>[4x]MRNKIFISHATPDDNDFTRWLALKLIGLGYEVWCDILFLDKGVDFWSNIEKVIREDTCKFLLVSSSYSNQREGVLKELAVAAKVKKQLKDDKFIIPLAIDEQLSYDDINIDIVRLNAIDFKMSWARGLKDILEAFEKQKVPKEVADASKSNLLYQQIFLHDKSVIEKEEIYDSNWLSILSFPEELRFHEYNWMLPKRFDVRELTFPAVRYKNYLCTFAWAYDFTYHLPKTETYHKSKTIRIPTEEILSGSYDSNFIRNAECKRLIVQLLNKAFELRMKDKEVQEYEMSNKTAYWLEKGKLEKDKFEKTMLVGKQKDKNWHFAISGASKLYPFPVLMISSHIFFTADGKKLIDSSSV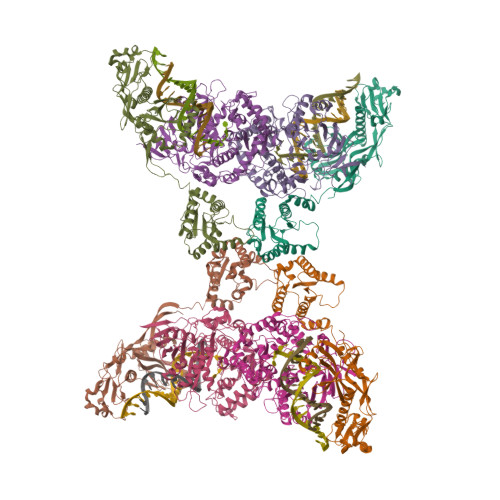QHSSRRRQGKNWWNNTWRTKLLAFIKYLSDDDTSFYLEMGSEEKVFVSNEPVKFKGNVSYNIPEKNTLEEEAELSGFNQGEDIEELEELIENLEAE;>MKELIYIEEPKILFAHGQKCTDARDGLALFGPLNNLYGIKSGVIGTKQGLKIFRDYLDHIQKPIYNSNSITRPMFPGFEAVFDCKWESTGITFKEVTNEDIGKFLYNSSTHKRTYDLVSLFIDKIISANKNEDENVDVWFVIVPDEIYKYCRPNSVLPKEMVQTKALMSKSKAKSFRYEPSLFPDINIELKEQEKEAETYNYDAQFHDQFKARLLKHTIPTQIFRESTLAWRDFKNAFGLPIRDFSKIEGHLAWTISTAAFYKAGGKPWKLSDVRNGVCYLGLVYKKVEKSKNPRNACCAAQMFLDNGDGTVFKGEVGPWYNPKNGQYHLEPKEAKALLSQSLQSYKEQIGEYPKEVFIHAKTRFNHQEWDAFLEVTPKETNLVGVTISKTKPLKLYKTEGDYTILRGNAYVVNERSAFLWTVGYVPKIQTALSMEVPNPLFIEINKGEADIKQVLKDILSLTKLNYNACIFADGEPVTLRFADKIGEILTASTDIKTPPLAFKYYI[4x]>MTKQYKNYVNGEWKLSENEIKIYEPASGAELGSVPAMSTEEVDYVYASAKKAQPAWRALSYIERAAYLHKVADILMRDKEKIGAILSKEVAKGYKSAVSEVVRTAEIINYAAEEGLRMEGEVLEGGSFEAASKKKIAVVRREPVGLVLAISPFNYPVNLAGSKIAPALIAGNVIAFKPPTQGSISGLLLAEAFAEAGLPAGVFNTITGRGSEIGDYIVEHQAVNFINFTGSTGIGERIGKMAGMRPIMLELGGKDSAIVLEDADLELTAKNIIAGAFGYSGQRSTAVKRVLVMESVADELVEKIREKVLALTIGNPEDDADITPLIDTKSADYVEGLINDANDKGATALTEIKREGNLICPILFDKVTTDMRLAWEEPFGPVLPIIRVTSVEEAIEISNKSEYGLQASIFTNDFPRAFGIAEQLEVGTVHINNKTQRGTDNFPFLGAKKSGAGIQGVKYSI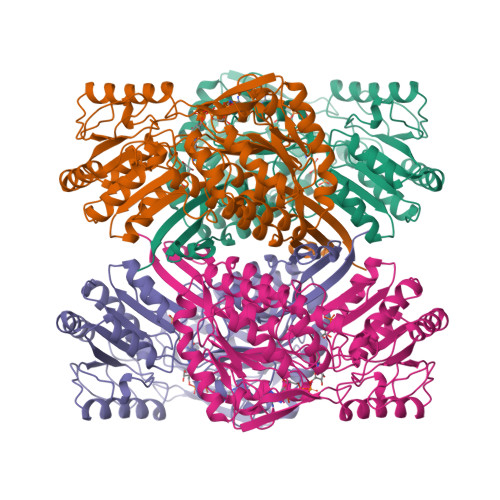EAMTTVKSVVFDIK[4x]> MSLTNDERILSWNETPSKPRYTPPPGAIDAHCHVFGPMAQFPFSPKAKYLPRDAGPDMLFALRDHLGFARNVIVQASCHGTDNAATLDAIARAQGKARGIAVVDPAIDEAELAALHEGGMRGIRFNFLKRLVDDAPKDKFLEVAGRLPAGWHVVIYFEADILEELRPFMDAIPVPIVIDHMGRPDVRQGPDGADMKAFRRLLDSREDIWFKATCPDRLDPAGPPWDDFARSVAPLVADYADRVIWGTDWPHP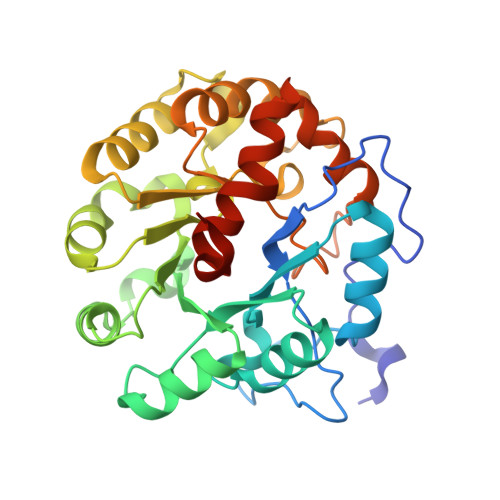NMQDAIPDDGLVVDMIPRIAPTPELQHKMLVTNPMRLYWSEEMEGHHHHHH> MAWPKVQPEVNIGVVGHVDHGKTTLVQAITGIWTSKHSEELKRGMTIKLGYAETNIGVCESCKKPEAYVTEPSCKSCGSDDEPKFLRRISFIDAPGHEVLMATMLSGAALMDGAILVVAANEPFPQPQTREHFVALGIIGVKNLIIVQNKVDVVSKEEALSQYRQIKQFTKGTWAENVPIIPVSALHKINIDSLIEGIEEYIKTPYRDLSQKPVMLVIRSFDVNKPGTQFNELKGGVIGGSIIQGLFKVDQEIKVLPGLRVEKQGKVSYEPIFTKISSIRFGDEEFKEAKPGGLVAIGTYLDPSLTKADNLLGSIITLADAEVPVLWNIRIKYNLLERVVGAKEMLKVDPIRAKETLMLSVGSSTTLGIVTSVKKDEIEVELRRPVAVWSNNIRTVISRQIAGRWRMIGWGLVEI

In eukaryotic and archaeal cells, the initiator tRNA carrier is the e/aIF2 heterotrimer. In its GTP-bound form, this factor specifically binds Met-tRNAiMet and brings it to the initiation complex. The γ subunit forms the core of the heterotrimer and contains the GTP-binding pocket. α and β are bound to γ but do not interact together. We were able to observe GTP hydrolysis by aIF2 or by its isolated γ subunit.

Comparison of the structure with the wt-aIF2γ-GDP-Mg2+ structure shows the transition between switch ON and switch OFF states. In the GDP-bound structure, the magnesium ion is still bound but three water molecules and one oxygen of the β phosphate define the equatorial plane, whereas another water molecule and the hydroxyl group of T23 are in apical positions with respect to Mg2+. Changes of the coordination of the magnesium ion are correlated to the structural change following the loss of the γ-phosphate previously termed the loaded-spring mechanism. Overall, the conformation of wt-aIF2γ−GDPNP differs from that of wt-aIF2γ-GDP by a rotation of domains II-III with respect to domain I by ca. 14°. This rotation is partly due to the movement of switch 2 helix, and to the subsequent remodeling of its interaction network with β17 and the following loop of domain III. In addition, transition of switch 1 position from ON to OFF causes release of interactions between domains I and II involving the strictly conserved R219 residue.> MDAPEEEDHVLVLRKSNFAEALAAHKYLLVEFYAPWCGHCKALAPEYAKAAGKLKAEGSEIRLAKVDATEESDLAQQYGVRGYPTIKFFRNGDTASPKEYTAGREADDIVNWLKKRTGPAATTLPDGAAAESLVESSEVAVIGFFKDVESDSAKQFLQAAEAIDDIPFGITSNSDVFSKYQLDKDGVVLFKKFDEGRNNFEGEVTKENLLDFIKHNQLPLVIEFTEQTAPKIFGGEIKTHILLFLPKSVSDYDGKLSNFKTAAESFKGKILFIFIDSDHTDNQRILEFFGLKKEECPAVRLITLEEEMTKYKPESEELTAERITEFCHRFLEGKIKPHLMSQELPEDWDKQPVKVLVGKNFEDVAFDEKKNVFVEFYAPWCGHCKQLAPIWDKLGETYKDHE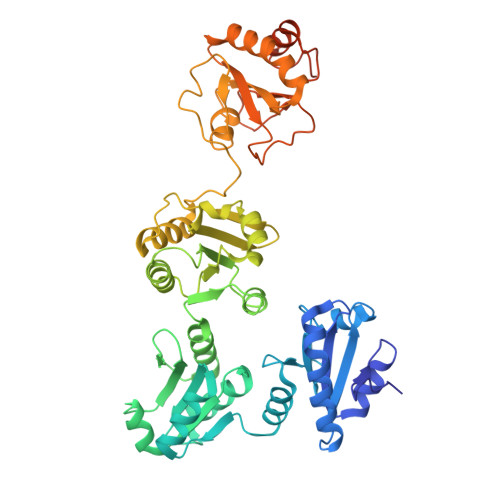NIVIAKMDSTANEVEAVKVHSFPTLKFFPASADRTVIDYNGERTLDGFKKFLESGGQDGAGDDDDLEDLEEAEEPDMEEDDDQKAVKDEL>[3x]MKKIEAIIRPFKLDEVKIALVNAGIVGMTVSEVRGFGRQKGQTERYRGAEYTVEFL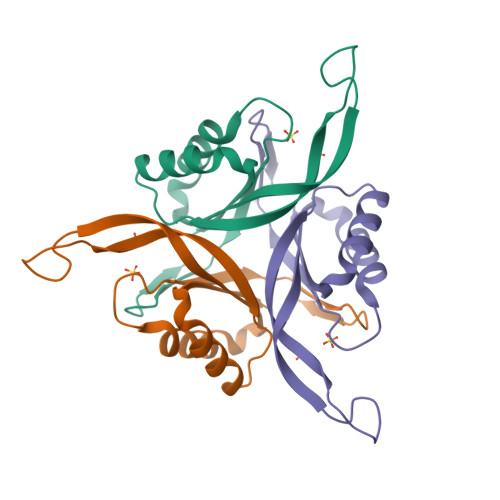QKLKLEIVVEDAQVDTVIDKIVAAARTGEIGDGKIFVSPVDQTIRIRTGEKNADAI>[2x]MASWSHPQFEKGASTSLYKKAGRMSKFTWKELIQLGSPSKAYESSLACIAHIDMNAFFAQVEQMRCGLSKEDPVVCVQWNSIIAVSYAARKYGISRMDTIQEALKKCSNLIPIHTAVFKKGEDFWQYHDGCGSWVQDPAKQISVEDHKVSLEPYRRESRKALKIFKSACDLVERASIDEVFLDLGRICFNMLMFDNEYELTGDLKLKDALSNIREAFIGGNYDINSHLPLIPEKIKSLKFEGDVFNPEGRDLITDWDDVILALGSQVCKGIRDSIKDILGYTTSCGLSSTKNVCKLASNYKKPDAQTIVKNDCLLDFLDCGKFEITSFWTLGGVLGKELIDVLDLPHENSIKHIRETWPDNAGQLKEFLD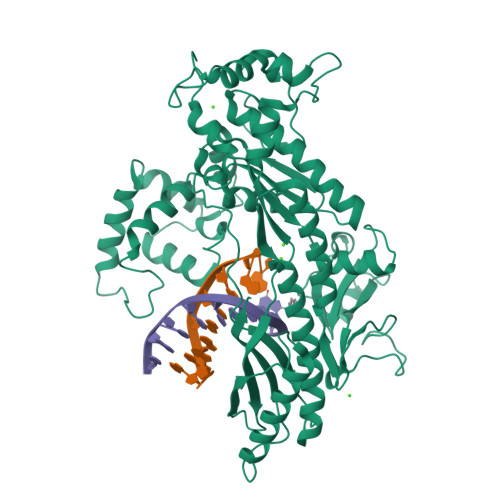AKVKQSDYDRSTSNIDPLKTADLAEKLFKLSRGRYGLPLSSRPVVKSMMSNKNLRGKSCNSIVDCISWLEVFCAELTSRIQDLEQEYNKIVIPRTVSISLKTKSYEVYRKSGPVAYKGINFQSHELLKVGIKFVTDLDIKGKNKSYYPLTKLSMTITNFDIIDLQK The human KCTD family contains 25 soluble proteins that share a conserved potassium (K+) Channel Tetramerization Domain (a subtype of ‘BTB domain’) at their N-termini and have variable C-termini. The BTB fold of the Kv and KCTD families has a roughly pyramidal wedge shape and consists of five α-helices and a single β-sheet made from three β-strands. Here, we present novel X-ray crystal structures of the BTB domains of a further five members of the KCTD family and examine the stoichiometry and stability of their multimeric assemblies in solution. Overall, the pyramidal wedge shape of the KCTD family BTB domain creates a versatile scaffold compatible with a range of oligomeric assemblies and geometries that may impact function.

KCTD10 is implicated in heart morphogenesis and congenital heart failure through regulation of Tbx5 and Notch1. In contrast, a novel tetrameric assembly with two-fold rotational symmetry is observed for both KCTD10 and KCTD13. A second interface is additionally evident in the tetrameric structures of KCTD10 and KCTD13 as visualized by an antiparallel arrangement of two β1–β2 hairpins. Whereas the canonical interface contributes 1210 Å2 to the total tetramer interface in KCTD10, the second interface contributes 940 Å2. For instance, the scattering curve for KCTD10 was virtually identical with that calculated for the two-fold symmetric tetramer observed in its crystal, while being distinct from the predicted solution scattering curve for a symmetric tetramer such as that observed for the T1 domain found attached to potassium channels. Interestingly, KCTD10 and KCTD13 also exhibited retention times and MALS scattering that were consistent with mixtures of monomers and dimers, indicating that these crystallographic tetramers were not stable in solution at lower protein concentrations (<50 µM monomer concentration compared with ∼750 µM used in SAXS experiments). Overall, the BTB domains displayed a range of affinities from low-to-high nanomolar: KCTD17 (Kd = 7 nM) > KCTD5 (Kd = 55 nM) > SHKBP1 (Kd = 87 nM) > KCTD13 (Kd = 100 nM), KCTD10 (Kd = 460 nM). Our crystal structures of KCTD10 and KCTD13 represent the first structures of family members from clade C. Unexpectedly, both proteins crystallized as two-fold symmetric tetramers revealing a different complex architecture to other KCTD families characterized to date. These structures were also notably distinct from the four-fold rotationally symmetric tetramer of the Kv4.3 BTB domain. It remains unclear if all KCTD family members would form KCTD5-like pentameric assemblies, or if for instance full-length KCTD10 or KCTD13, which belong to a relatively diverged clade, would retain tetrameric forms similar to their isolated BTB domain structures.

>SMGTSPSSKYVKLNVGGALYYTTMQTLTKQDTMLKAMLSGRMEVLTDSEGWILIDRCGKHFGTILNYLRDGAVPLPESRREIEELLAEAKYYLVQGLVEECQAALQNKDTYE[4x]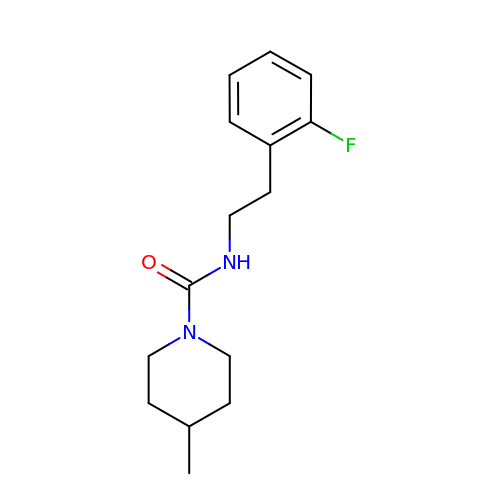~{N}-[2-(2-fluorophenyl)ethyl]-4-methyl-piperidine-1-carboxamide | C15 H21 F N2 O | ZOWZHYQKQARZGD-UHFFFAOYSA-N> PIFLNVLEAIEPGVVCAGHDNNQPDSFAALLSSLNELGERQLVHVVKWAKALPGFRNLHVDDQMAVIQYSWMGLMVFAMGWRSFTNVNSRMLYFAPDLVFNEYRMHKSRMYSQC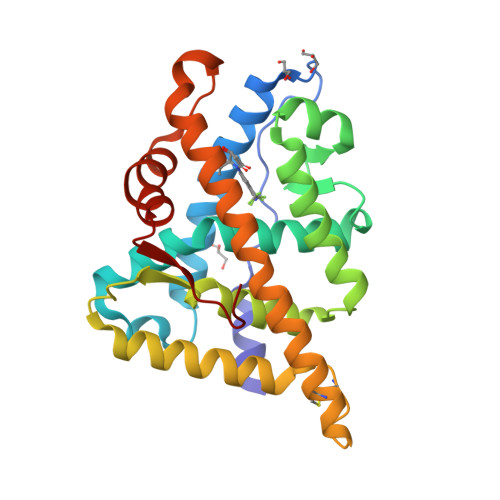VRMRHLSQEFGWLQITPQEFLCMKALLLFSIIPVDGLKNQKFFDELRMNYIKELDRIIACARKNPTSCSRRFYQLTKLLDSVQPIARELHQFTFDLLIKSHMVSVDFPEMMAEIISVQVPKILSGKVKPIYFHTQ>[2x]MTATDNARQVTIIGAGLAGTLVARLLARNGWQVNLFE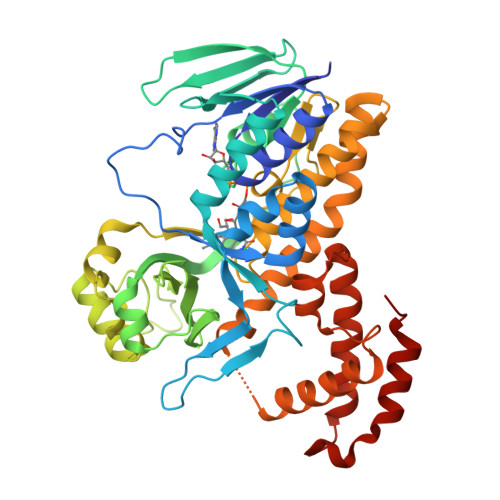RRPDPRIETGARGRSINLALAERGAHALRLAGLEREVLAEAVMMRGRMVHVPGTPPNLQPYGRDDSEVIWSINRDRLNRILLDGAEAAGASIHFNLGLDSVDFARQRLTLSNVSGERLEKRFHLLIGADGCNSAVRQAMASVVDLGEHLETQPHGYKELQITPEASAQFNLEPNALHIWPHGDYMCIALPNLDRSFTVTLFLHHQSPAAQPASPSFAQLVDGHAARRFFQRQFPDLSPMLDSLEQDFEHHPTGKLATLRLTTWHVGGQAVLLGDAAHPMVPFHGQGMNCALEDAVALAEHLQSAADNASALAAFTAQRQPDALAIQAMALENYVEMSSKVASPTYLLERELGQIMAQRQPTRFIPRYSMVTFSRLPYAQAMARGQIQEQLLKFAVANHSDLTSINLDAVEHEVTRCLPPLSHLS>MTENTKNENITNILTQKLIDTRTVLIYGEINQELAEDVSKQLLLLESISNDPITIFINSQGGHVEAGDTIHDMIKFIKPTVKVVGTGWVAAAGITIYLAAEKENRFSLPNTRYMIHQPAGGVQGQSTEIEIEAKEIIRMRERINRLIAEATGQSYEQISKDTDRNFWLSVNEAKDYGIVNEIIENRDGLK[7x];>MNLIPTVIEQTSRGERAYDIYSRLLKDRIIMLGSAIDDNVANSIVSQLLFLDAQDPEKDIFLYINSPGGSISAGMAIYDTMNFVKADVQTIGMGMAAAMGSFLLTAGANGKRFALPNAEIMIHQPLGGAQGQATEIEIAARHILKIKE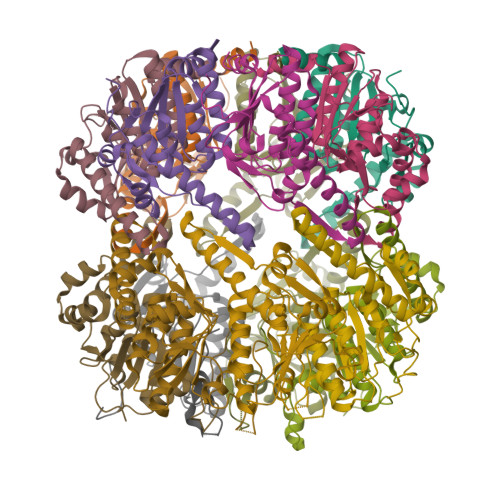RMNTIMAEKTGQPYEVIARDTDRDNFMTAQEAKDYGLIDDIIINKSGLKG[7x]> MPKTISVRVTTMDAELEFAIQPNTTGKQLFDQVVKTIGLREVWFFGLQYQDTKGFSTWLKLNKKVTAQDVRKESPLLFKFRAKFYPEDVSEELIQDITQRLFFLQVKEGILNDDIYCPPETAVLLASYAVQSKYGDFNKEVHKSGYLAGDKLLPQRVLEQHKLNKDQWEERIQVWHEEHRGMLREDAV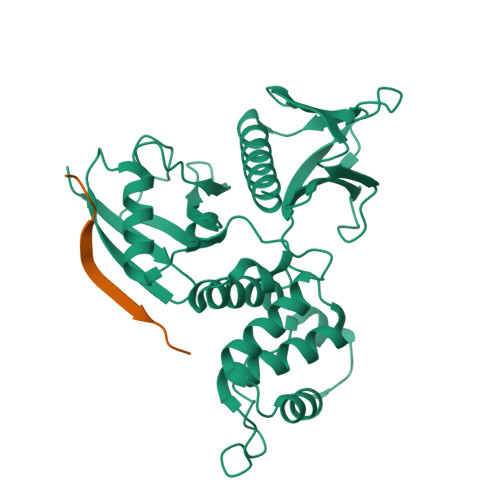LEYLKIAQDLEMYGVNYFSIKNKKGSELWLGVDALGLNIYEQNDRLTPKIGFPWSEIRNISFNDKKFVIKPIDKKAPDFVFYAPRLRINKRILALCMGNHELYMRRRK;> DSEPVLKGVKLHYT> HHHHHHHMMDQQSTRTDITVNVDGFWMLQALLDIRHVAPELRCRPYVSTDSNDWLNEHPGMAVMREQGIVVNDAVNEQVAARMKVLAAPDLEVVALLSRGKLLYGVIDDENQPPGSRDIPDNEFRVVLARRGQHWV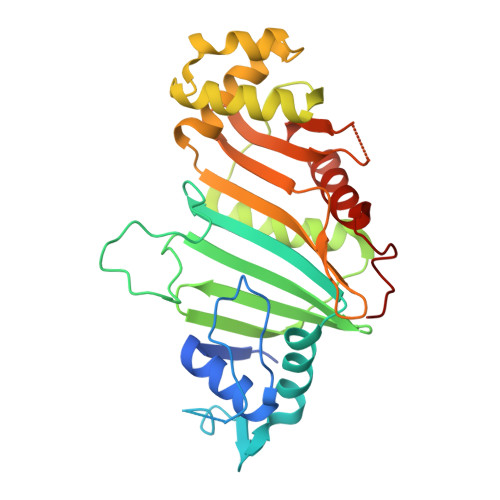SAVRVGNDITVDDVTVSDSASIAALVMDGLESIHHADPAAINAVNVPMEEMLEATKSWQESGFNVFSGGDLRRMGISAATVAALGQALSDPAAEVAVYARQYRDDAKGPSASVLSLKDGSGGRIALYQQARTAGSGEAWLAICPATPQLVQVGVKTVLDTLPYGEWKTHSRV>[4x]GSLDGPYAPDSSNLPSNC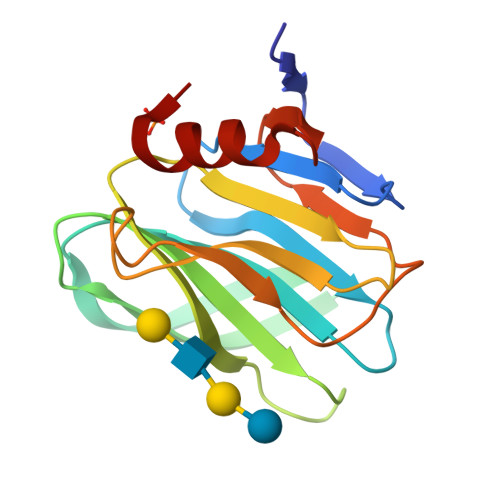WYLVNPSNDGVVFSVTDNSTFWMFTYLVLPNTAQTNVTVNVMNETVNISIDNSGSTYRFVDYIKTSSTQAYGSRNYLNTAHRLQAYRRDGDGNISNYWGADTQGDLRVGTYSNPVPNAVINLNADFYVIPDSQQETCTEYIRGGL> MKVFDVHKFDMKKEQDFLQVQFNLKNRINLSPTIHPDSINTTAGVDLAYWEQDGEPYGVCCII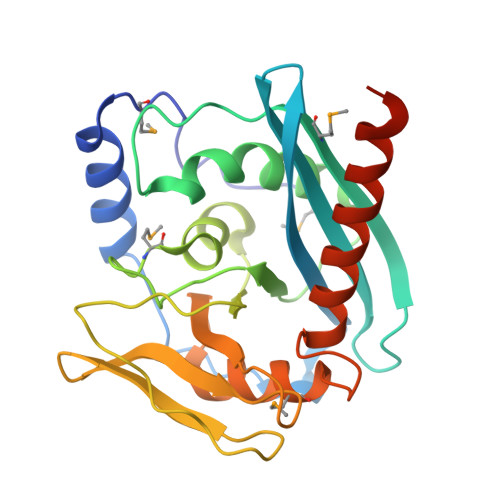VIDADTKEVIEKVHSMGRISVPYVSGFLAFRELPLIIEAAKKLETEPDVFLFDGNGYLHYNHMGVATHAAFFLGKPTIGIAKTYLKIKGCDFVTPEIEVGAYTDIIIDGEVYGRALRTRRDVKPIFLSCGNYIDLDSSYQITMSLINQESRLPIPVRLADLETHVLRTFYQKNHVLEHHHHHH Paraherquamide A | C28 H35 N3 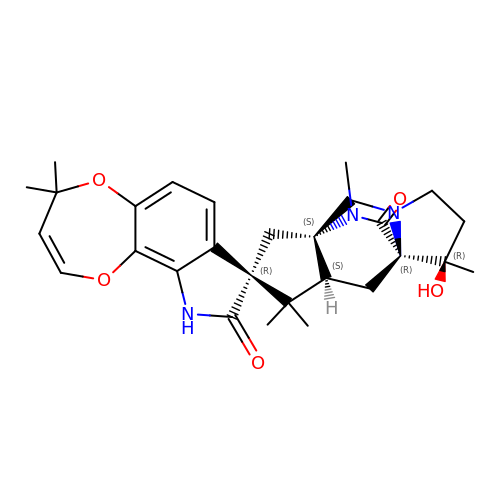O5 | UVZZDDLIOJPDKX-ITKQZBBDSA-N1-(2-{4-[(4aS,8aR)-4-(3,4-dimethoxyphenyl)-1-oxo-1,2,4a,5,8,8a-hexahydrophthalazin-2-yl]piperidin-1-yl}-2-oxoethyl)pyrrolidine-2,5-dione | C27 H32 N4 O6 | 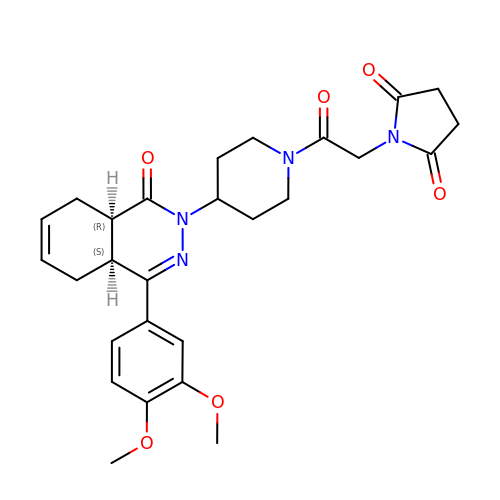BLRZNXZBGGTDMQ-VQTJNVASSA-N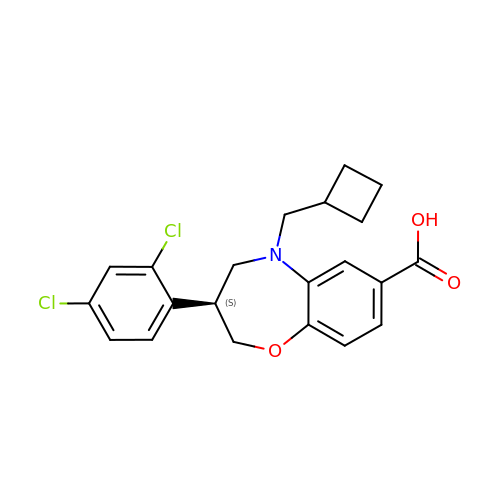(3S)-5-(cyclobutylmethyl)-3-(2,4-dichlorophenyl)-2,3,4,5-tetrahydro-1,5-benzoxazepine-7-carboxylic acid | C21 H21 Cl2 N O3 | FLTAOBQLOVJBJL-HNNXBMFYSA-N The utility of this method is illustrated by way of an XP Screen against CYP121A1, a cytochrome P450 enzyme from Mycobacterium tuberculosis (Mtb) championed as a validated drug discovery target. CYP121A1 (mycocyclosin synthase; EC 1.14.19.70; Rv2276), functioning downstream of the cyclo(l-tyrosyl-l-tyrosyl) (cYY) synthase (EC 2.3.2.21; Rv2275), catalyzes the conversion in Mtb of the cyclic dipeptide cYY into the highly strained biaryl-containing natural product mycocyclosin. Whilst the precise function of mycocyclosin remains unknown, ablation of CYP121A1 expression via genetic knockouts showed the enzyme to be essential for the viability of the bacterium in vitro; CYP121A1 is thus seen as an important target for anti-TB drug research. The CYP121A1 binding pocket has been shown by X-ray crystallography to accommodate ligands in three distinct regions (i) binding to the heme group, (ii) binding in the cYY region and (iii) binding at the top of the binding pocket.

Compounds 4–37 were screened crystallographically against CYP121A1 using soaking experiments. A number of hits (7, 10, 14, 21, 31 and 33) were identified, although the completeness of the electron density for the ligands was variable. All six of the X-ray crystallographic hits were ligands containing 7 as an integral subunit of molecular structure. X-ray crystal structures of compounds 10 and 21 with CYP121A1, whilst of better quality, still suffered from incomplete ligand electron density, either lacking complete density for the indole moiety (for 10) or lacking density for the central linker (for 21). Hydrogenation of 11 over palladium on carbon in ethanol in the presence of triethylamine yielded the known pyrimidine 10. Most compounds gave inconclusive results as a result of aggregation, due to limited ligand solubility in the aqueous buffer. Compounds with lower cLogP proved to be less problematic, with both 10 (an X-ray hit) and 55 (the 5-hydroxy derivative of the key X-ray hit 14) also showing evidence of activity (protein melting temperature shifts of +3.5 °C and +0.5 °C respectively).

> MTATVLLEVPFSARGDRIPDAVAELRTREPIRKVRTITGAEAWLVSSYALCTQVLEDRRFSMKETAAAGAPRLNALTVPPEVVNNMGNIADAGLRKAVMKAITPKAPGLEQFLRDTANSLLDNLITEGAPADLRNDFADPLATALHCKVLGIPQEDGPKLFRSLSIAFMSSADPIPAAKINWDRDIEYMAGILENPNITTGLMGELSRLRKDPAYSHVSDELFATIGVTFFGAGVISTGSFLTTALISLIQRPQLRNLLHEKPELIPAGVEELLRINLSFADGLPRLATADIQVGDVLVRKGELVLVLLEGANFDPEHFPNPGSIELDRPNPTSHLAFGRGQHFCPGSALGRRHAQIGIEALLKKMPGVDLAVPIDQLVWRTRFQRRIPERLPVLW>MSIEKLKAALPEYAKDIKLNLSSITRSSVLDQEQLWGTLLASAAATRNPQVLADIGAEATDHLSAAARHAALGAAAIMGMNNVFYRGRGFLEGR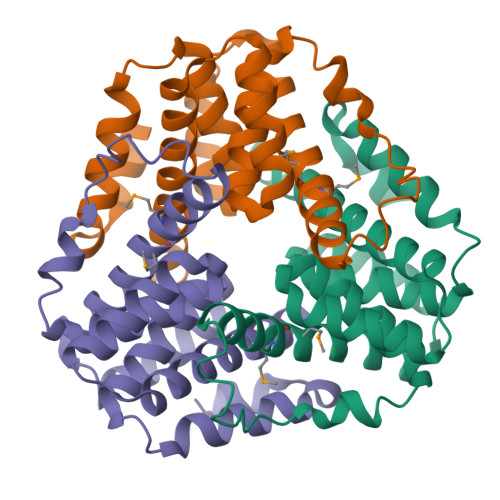YDDLRPGLRMNIIANPGIPKANFELWSFAVSAINGCSHCLVAHEHTLRTVGVDREAIFEALKAAAIVSGVAQALATIEALSPS[12x]> MGSSHHHHHHSSGLVPRGSGSDPTRKQKVEAQKQAEKLMKQIGVKNVKLSEYEMSIAAHLVDPLNMHVTWSDIAGLDDVITDLKDTVILPIKKKHLFENSRLLQPPKGVLLYGPPGCGKTLIAKATAKEAGCRFINLQPSTLTDKWYGESQKLAAAVFSLAIKLQPSIIFIDQIDSFL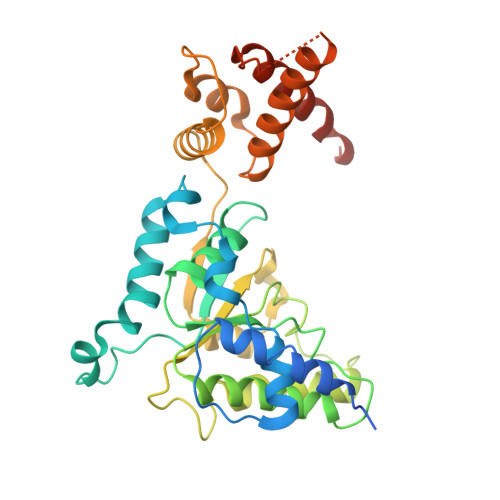RNRSSSDHEATAMMKAQFMSLWDGLDTDHSCQVIVMGATNRPQDLDSAIMRRMPTRFHINQPALKQREAILKLILKNENVDRHVDLLEVAQETDGFSGSDLKEMCRDAALLCVREYVNSTSEESHDEDEIRPVQQQDLHRAIEKMKKSKDAAFQNVLTHVCLD>MKLKTTLFGNVYQFKDVKEVLAKANELRSGDVLAGVAAASSQERVAAKQVLSEMTVADIRNNPVIAYEDDCVTRLIQ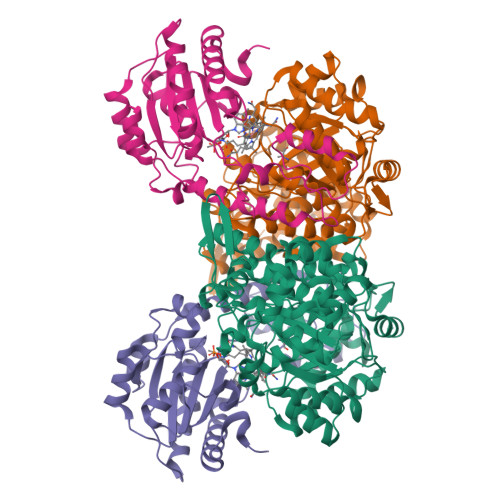DDVNETAYNQIKNWSISELREYVLSDETSVDDIAFTRKGLTSEVVAAVAKICSNADLIYGAKKMPVIKKANTTIGIPGTFSARLQPNDTRDDVQSIAAQIYEGLSFGVGDAVIGVNPVTDDVENLSRVLDTIYGVIDKFNIPTQGCVLAHVTTQIEAIRRGAPGGLIFQSICGSEKGLKEFGVELAMLDEARAVGAEFNRIAGENCLYFETGQGSALSAGANFGADQVTMEARNYGLARHYDPFIVNTVVGFIGPEYLYNDRQIIRAGLEDHFMGKLSGISMGCDCCYTNHADADQNLNENLMILLATAGCNYIMGMPLGDDIMLNYQTTAFHDTATVRQLLNLRPSPEFERWLESMGIMANGRLTKRAGDPSLFF[2x];>[2x]MDQSSHHHHHHALDLGSAEAKAWIGVENPHRADVLTELRRSTVARVCTGRAGPRPRTQALLRFLADHSRSKDTVLKEVPEEWVKAQGLLEVRSEISDKNLYLTRPDMGRRLCAEAVEALKAQCVANPDVQVVISDGLSTDAITVNYEEILPPLMAGLKQAGLKVGTPFFVRYGRVKIEDQIGEILGAKVVILLVGERPGLGQSESLSCYAVYSPRMATTVEADRTCISNIHQGGTPPVEAAAVIVDLAKRMLEQKASGINMTR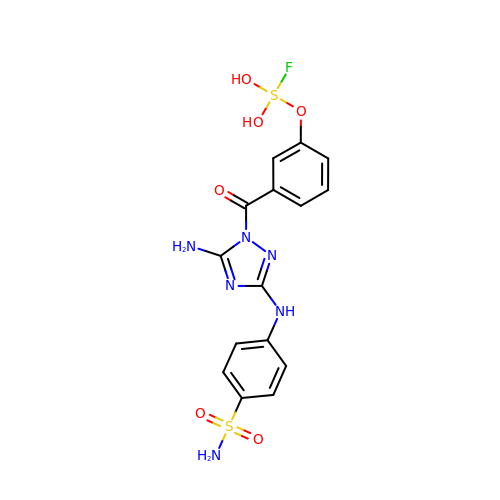4-{[5-amino-1-(3-{[fluorodi(hydroxy)-lambda~4~-sulfanyl]oxy}benzoyl)-1H-1,2,4-triazol-3-yl]amino}benzene-1-sulfonamide | C15 H15 F N6 O6 S2 | VNMSMWQDKZDYKK-UHFFFAOYSA-N>[2x]MGLLSILRKLKSAPDQEVRILLLGLDNAGKTTLLKQLASEDISHITPTQGFNIKSVQSQGFKLNVWDIGGQRKIRPYWRSYFENTDILIYVIDSADRKRFEETGQELTELLEEEKLSCVPVLIFANKQDLLTAAPASEIAEGLNLHTIRDRVWQIQSCSALTGEGVQDGMNWVCKNVNAKKKLEHHHHHH;>[2x]GPMAAEEEDEVEWVVESIAGFLRGPDWSIPILDFVEQKCEVFDDEEESKLTYTEIHQEYKELVEKLLESYLKEIGINEDQFQEACTSPLAKTRTSQAILQPVLAAEDFTIFKAMMVQKNIEMQLQAIRIIQERNG

The ciliary protein Arl3 has been shown to act as a specific release factor for myristoylated and farnesylated ciliary cargo molecules by binding to the effectors Unc119 and PDE6δ. Here we describe a newly identified Arl3 binding partner, CCDC104/CFAP36. Biochemical and structural analyses reveal that the protein contains a BART-like domain and is called BARTL1. It recognizes an LLxILxxL motif at the N-terminal amphipathic helix of Arl3, which is crucial for the interaction with the BART-like domain but also for the ciliary localization of Arl3 itself.

Here, we demonstrate by X-ray structure determination that BARTL1 binds Arl3∙GppNHp in a similar fashion to BART complexing Arl2∙GTP (Zhang et al., 2009). The asymmetric unit contained two Arl3∙GppNHp and two BARTL1133 molecules. BARTL1133 displays the same all-helical fold as seen in BART (Zhang et al., 2009). As expected for an effector of small G proteins, BARTL1 is in contact with the switch regions of Arl3 (area 2). In addition, BARTL1 completely buries the N-terminal helix of Arl3 (area 1). This unconventional binding mode sets it apart from effectors such as PDE6δ or Unc119 and from many other effectors of the Ras superfamily proteins. The hydrophobic side of the N-terminal amphipathic helix of Arl3 is buried in a hydrophobic groove formed by helices α3, α4, α4′, and α5 of BARTL1. Leu3A, Leu4A, Ile6A, Leu7A, and Leu10A are submerged in a hydrophobic patch made up by Lys58B, Val61B, Leu65B, and Leu69B on α3, Phe79B and Cys83B on α4, Ala88B on α4′, and Leu97B, Val100B, and Leu101B on α5 (BARTL1 [B] and Arl3 [A]; Figures 4A area 1, and 4B). The second interface area is formed by switch I, switch II, and residues of the interswitch toggle of Arl3, and on the BARTL1133 side by the loop connecting α2 and α3 as well as parts of the α3 and α6 helices (area 2). There are polar interactions between Thr51B and Tyr81A, switch I main-chain nitrogens of Gln49A and Gly50A with Glu45B and Glu44B of the α2-α3 loop with Lys45A of β2 in the interswitch toggle and Lys35A in the α1 helix.1,3,5(10)-ESTRATRIEN-2,3,17-BETA-TRIOL 2-METHYL ETHER | C19 H26 O3 | 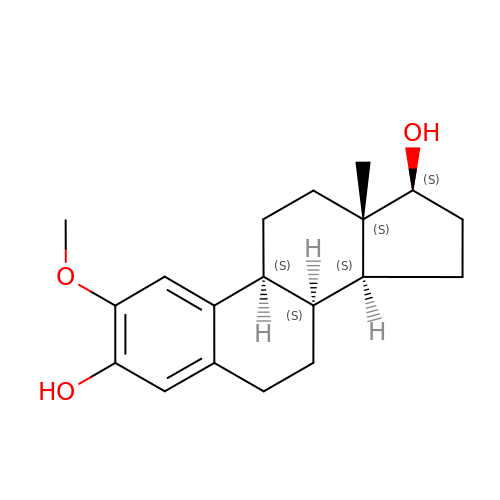CQOQDQWUFQDJMK-SSTWWWIQSA-N> MDAAEVEFLAEKELVTIIPNFSLDKIYLIGGDLGPFNPGLPVEVPLWLAINLKQRQKCRLLPPEWMDVEKLEKMRDHERKEETFTPMPSPYYMELTKL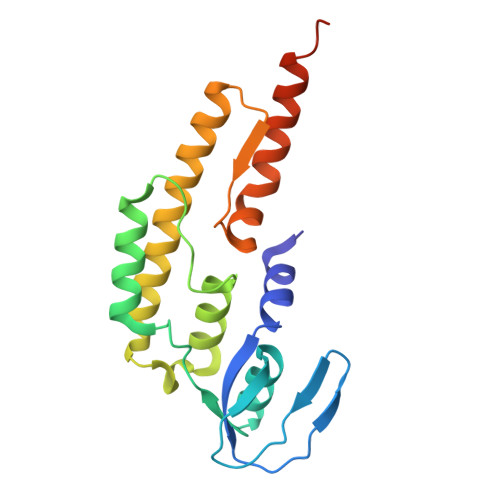LLNHASDNIPKADEIRTLVKDMWDTRIAKLRVSADSFVRQQEAHAKLDNLTLMEINTSGTFLTQALNHMYKLRTNLQPLESTQSQDF>[2x]MKKPRIDMHSHFFPRISEQEAAKFDANHAPWLQVSAKGDTGSIMMGKNNFRPVYQALWDPAFRIEEMDAQGVDVQVTCATPVMFGYTWEANKAAQWAERM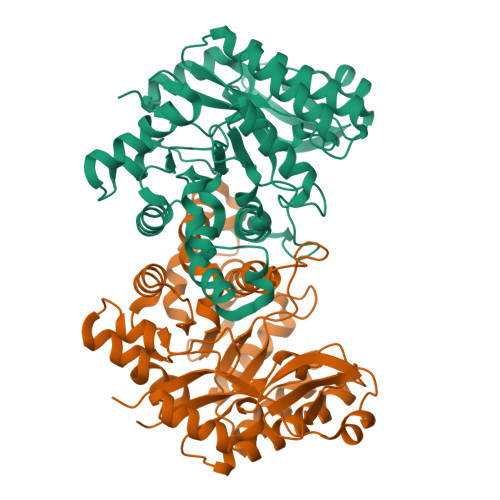NDFALEFAAHNPQRIKVLAQVPLQDLDLACKEASRAVAAGHLGIQIGNHLGDKDLDDATLEAFLTHCANEDIPILVHPWDMMGGQRMKKWMLPWLVAMPAETQLAILSLILSGAFERIPKSLKICFGHGGGSFAFLLGRVDNAWRHRDIVREDCPRPPSEYVDRFFVDSAVFNPGALELLVSVMGEDRVMLGSDYPFPLGEQKIGGLVLSSNLGESAKDKIISGNASKFFNINV>MSGSPAPQGALRQRIVASTPKKTKESKDGAASDAELDKLVKEAAAAKAPAGSERDYKIAFAIITALAFLTRFWGISHPDQVVFDEVHFGKFASYYLQRTYFFDVHPPLGKLLFAFMGWLVGYDGHFHFDNIGDPYVINKVPYVAFRALPAILGSLTVSVVFLIMWESGYSLPACILASGLVLLDNAHIGQTRLILLDATLVFAMACSLLCYIKFYKLRHEPFSRKWWKWLILTGFALSCDISTKYVGLFAFITIGSAVCIDLWDLLNINRPKGALTLPQFGKHFAARAFGLIFMPFMFYLFWFQVHFSILTRSGPGDDFMTPEFQETLSDNIMLANAVTIDYWDTITIKHKETKAYLHSHPDRYPLRYDDGRVSSQGQQVTGYPFNDTNNWWQILPAGPFEEPKLGRHVKHRDLVRLRHVGTDTYLLSHDVASPYYPTNQEFTTVSFNEAYGDRAADTLFEVRIEHGKPGQEFKSISSHFKLIHNPSKVAMWTHPTPLPDWGHRQQEINGNKQIAPSSNVWLVEDIVSLPADHKRREKPERKVKTLPFLRKWFELQRSMFWHNNQLTASHPYASLPYQWPFLLRGVSFWTNSETRQQIYFLGNPVGWWIASSVLAIYVGIVLADQFSLRRGIDALDHRTRSRLYNSTGFFFLAWATHYFPFFVMGRQLFLHHYLPAHLASTLVTGALVEFIFSPEAPEHEIAAQQAKSSSSGKRGGVAMKRHITARERFAGQSLMGSWIATAVILALVAWSWWFFLPLTYGYPGMSVQQVLRRKWLGYDLHFAKLEVLFQGPGSHHHHHHHHHH[2x]

Protein O-mannosyltransferases (PMTs) are conserved endoplasmic reticulum membrane-embedded enzymes responsible for the transfer of mannose from dolichol phosphate-mannose (Dol-P-Man) to serine/threonine-rich protein substrates or unfolded proteins. PMTs from three subfamilies form obligate dimers with different substrate specificities and require the concerted action of their transmembrane domains (TMDs) and a luminal MIR domain for catalysis. Here, we present structures, native mass spectrometry, and structure-based mutagenesis of the fungal Pmt4 homodimer. The core fold of the TMDs and MIR domain is conserved with the Pmt1-Pmt2 heterodimer, indicating a shared catalytic mechanism.

Structural analysis by single-particle cryo-electron microscopy (cryo-EM) confirmed ctPmt4 is a homodimer, allowing processing of the data with either no symmetry (C1) or two-fold rotational symmetry (C2) imposed. In contrast, the luminal MIR domains were arranged asymmetrically and only resolved in the C1 reconstruction at a resolution that precluded direct model building. Therefore, we purified the ctPmt4-MIR domain from Escherichia coli via a N-terminal hexa-histidine tag and solved the crystal structure at 1.2 Å resolution by molecular replacement. Our final composite model for the ctPmt4 homodimer was derived from rigid body fitting these high-resolution structures for the TMDs and MIR domain into the C1 reconstruction and directly building models for their connecting linkers into the remaining density. The luminal MIR domains of ctPmt4 adopt a strikingly different arrangement with respect to the TMDs, compared to within the scPmt1-Pmt2 heterodimer; whilst the scPmt1- and scPmt2-MIR domains are positioned to interact in trans with the TMDs of the opposing dimer subunit, the first ctPmt4-MIR domain is rotated by 30o relative to the membrane and consequently interacts in cis with the TMDs from the same dimer subunit. Interestingly, whilst the second ctPmt4-MIR domain is also positioned in cis, it is rotated a further 30o so that it no longer interacts with the TMDs, akin to the scPmt2-MIR domain. Therefore, despite major differences in the cis/trans nature of their interactions, the MIR domains of both the ctPmt4 homodimer and scPmt1-Pmt2 heterodimer have a similar asymmetric arrangement, whereby one MIR domain is attached to the TMDs and the other is detached from them. In the attached ctPmt4 TMD-MIR interface, the active site is completely covered by this δ site, whilst in the detached conformation, the MIR domain is rolled aside and the active site is fully accessible. Instead, the attached MIR domain directly contacts the TMDs via the β8−β9 loop, whereby exposed histidine and charged residues (E465, H466, K468) form a relatively weak interface with aromatic residues of the TMDs (F319, H561, W562).>SMANLRKVLISDSLDPCCRKILQDGGLQVVEKQNLSKEELIAELQDCEGLIVRSATKVTADVINAAEKLQVVGRAGTGVDNVDLEAATRKGILVMNTPNGNSLSAAELTCGMIMCL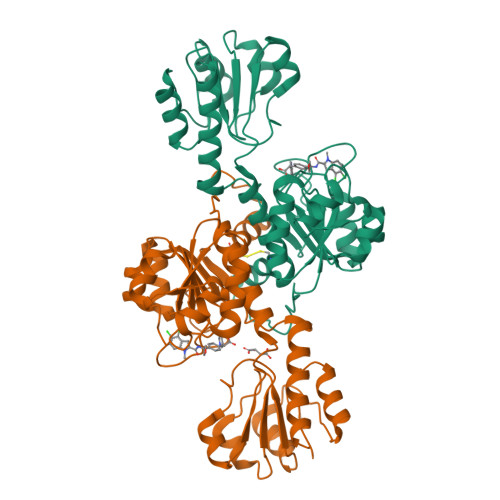ARQIPQATASMKDGKWERKKFMGTELNGKTLGILGLGRIGREVATRMQSFGMKTIGYDPIISPEVSASFGVQQLPLEEIWPLCDFITVHTPLLPSTTGLLNDNTFAQCKKGVRVVNCARGGIVDEGALLRALQSGQCAGAALDVFTEEPPRDRALVDHENVISCPHLGASTKEAQSRCGEEIAVQFVDMVKGKSLTGV[8x]>MATQEEILDAALVSGDSSQLTDSHLVALRLQQQVERIRQTRTQLLDGLYQNLSQAYDPGAASMWVLPANPDNTLPFLIGDKGRVLASLSLEAGGRGLAYGTNVLTQLSGTNAAHAPLLKRAVQWLVNGDPGAATAKDFKVSVVGVDKTAALNGLKSAGLQPADAACNALTDASCASTSKLLVLGNGASAASLSATVRARLQAGLPILFVHTNGWNQSSTGQQILAGLGLQEGPYGGNYWDKDRVPSSRTRTRSVELGGAYGQDPALVQQIVDGSWRTDYDWSKCTSYVGRTTCDDVPGLSDFSKRVDVLKGALDAYNQKAQNLFALPGTTSLRLWLLWADAVRQNIRYPMDKAADTARFQETFVADAIVGYVREAGAAQKELGSYAGQRQQSMPVSGSEETLTLTLPSAQGFTAIGRMAAPGKRLSIRIEDAGQASLAVGLNTQRIGSTRLWNTRQYDRPRFLKSPDIKLQANQSVALVSPYGGLLQLVYSGATPGQTVTVKVTGAASQPFLDIQPGEDSSQAIADFIQALDADKADWLEIR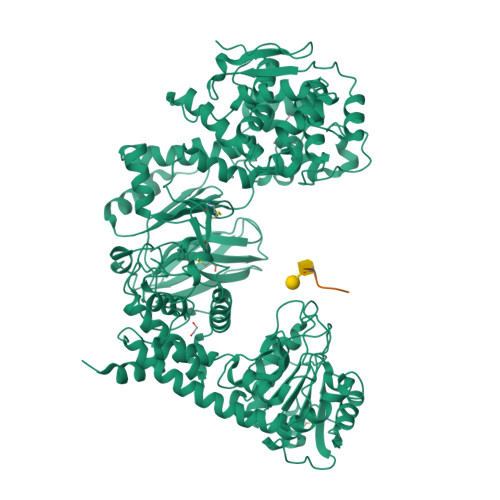SGSVEVHAKVEKVRGSIDKDYGGDVQRFIRELNEVFIDDAYTLAGFAIPNQAKTPAIQQECAARGWDCDSETLHKLPGTQHINVDQYAQCGGGCSGNPYDQTWGLNPRGWGESHQLGHNLQVNRLKVYGGRSGEISNQIFPLHKDWRVLREFGQNLDDTRVNYRNAYNLIVAGRAEADPLAGVYKRLWEDPGTYALNGERMAFYTQWVHYWADLKNDPLQGWDIWTLLYLHQRQVDKSDWDANKAALGYGTYAQRPGNSGDASSTDGNDNLLLGLSWLTQRDQRPTFALWGIRTSAAAQAQVAAYGFAEQPAFFYANNRTNEYSTVKLLDMSQGSPAWPFPLE[2x];>[2x]GAEAEAPSAVPDAAG>[2x]MDHLPIFCQLRDRDCLIVGGGDVAERKARLLLEAGARLTVNALTFIPQFTVWANEGMLTLVEGPFDETLLDSCWLAIAATDDDTVNQRVSDAAESRRIFCNVVDAPKAASFIMPSIIDRSPLMVAVSAGGTSHVLARLLREKLESLLPQHLGQVARYAGQLRARVKKQFATMGERRRFWEKFFVNDRLAQSLANADEKAVNATTERLFSEPLDHRGEVVLVGAGPGDAGLLTLKGLQQIQQADIVVYDRLVSDDIMNLVRRDADRVFVGKRAGYHCVPQEEINQILLREAQKGKRVVRLKGGDPFIFGRGGEELETLCHAGIPFSVVPGITAASGCSAYSGIPLTHRDYAQSVRLVTGHLKTGGELDWENLAAEKQTLVFYMGLNQAATIQEKLIAFGMQADMPVALVENGTSVKQRVVHGVLTQLGELAQQVESPALIIVGRVVALRDKLNWFSNH

Siroheme is the modified isobacteriochlorin tetrapyrrole used by siroheme-dependent sulfite and nitrite reductases (SiR/NiRs) in catalyzing the six-electron reduction of sulfite to sulfide or nitrite to ammonia. CysG is encoded by a gene fusion between a C-terminal SUMT (CysGA) and an N-terminal bifunctional dehydrogenase/ferrochelatase (CysGB). The N-terminal enzyme module, CysGB, is a three-domain bifunctional dehydrogenase/ATP-independent class III ferrochelatase12 that performs the final two steps of siroheme biosynthesis. The C-terminal enzyme module, CysGA, is homologous to a well-studied class of SAM-dependent uro’gen III methyltransferases (SUMTs) that catalyzes the methylations to generate precorrin-210,13.

P1331Cβ sits 3.3 Å below the plane formed by the sirohydrochlorin isobacteriochlorin core, forming a hydrophobic platform for the macrocycle. Both P133G and P133H variants retained the ability to complement the cysG-deficient E. coli when challenged for growth on minimal media, albeit with accumulation of fluorescence indicating altered activity. The P133G variant has 5-fold lower dehydrogenase activity and is about 10-fold lower in its chelatase activity, whereas the P133H variant is deficient for dehydrogenase activity and about 10-fold lower in its chelatase activity. Structurally, the histidine side chain projects in the active site, where it would interfere with tetrapyrrole binding, but no gross structural defects were present in the P133H variant as evidenced by a low RMSD to Met8p. The bulkier histidine projects into the active site, positioned in place of the pyrrole nitrogens when the tetrapyrrole binds, so would also disrupt tetrapyrrole binding and release. P133H behaves similarly to R260A, somewhat less sensitive.4-[5-(1,3-benzodioxol-5-yl)-4-(pyridin-2-yl)-1H-imidazol-2-yl]benzamide | C22 H16 N4 O3 | 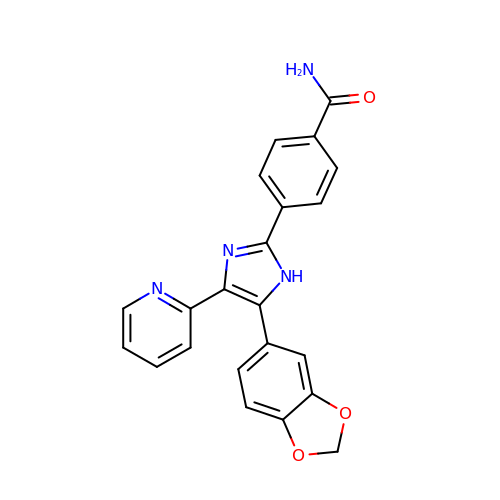FHYUGAJXYORMHI-UHFFFAOYSA-N>GAMGNKEQKNNNNVKEVSDSVQEDGLNDLYNNQEKQKSFTKNFGERKYEDLINPIEPIIPSESPKNKANIPNISIAHTEKKETKKENLIPSTNEEKEADAAIKYLEENILKNSKFSELIREVRVIKDEYALIKADLYDVIGKINNKKTSLMENPK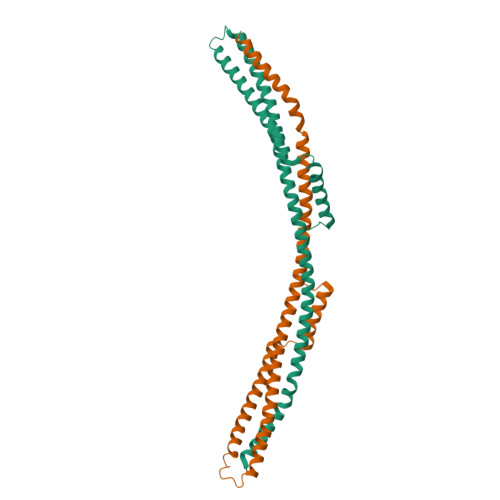NNRDKINKLTQLLQNNLKIDSELEQLINMIDMAENEISSAAFFFDNAQKRLKESIIKRLESKNNRSYALKLSRQALSDARSALSNLESFASKRIEPMVRKEEIKELIKHAKTVLESLNKK[2x]>GSMDFSRNLYDIGEQLDSEDLASLKFLSLDYIPQRKQEPIKDALMLFQRLQEKRMLEESNLSFLKELLFRINRLDLLITYLNTRKEEMERELQTPGRAQISAYRVMLYQISEEVSRSELRSF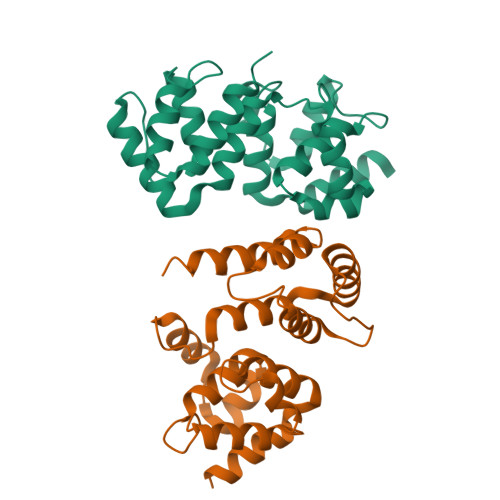KALLQEEDSKCKLDDDMNLLDIFIEMEKRVILGEGKLDILKRVCAQINKSLLKIINDYEEFSKERSSS[2x]>MKEGKHFVLVHGACHGGWSWYKLKPLLEAAGHKVTALDLAASGTDLRKIEELRTLYDYTLPLMELMESLSADEKVILVGHSLGGMNLGLAMEKYPQKIYAAVFLAAFMPDSVHNSSFVLEQ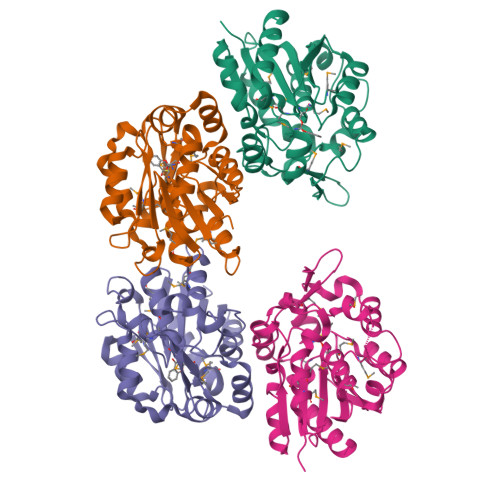YNERTPAENWLDTQFLPYGSPEEPLTSMFFGPKFLAHKLYQLCSPEDLALASSLVRPSSLFMEDLSKAKYFTDERFGSVKRVYIVCTEDKGIPEEFQRWQIDNIGVTEAIEIKGADHMAMLCEPQKLCASLLEIAHKYNMAGDPLEHHHHHH[4x]> SHMPIQVLPPQLANQIAAGEVVERPASVVKELVENSLDAGATRIDIDIERGGAKLIRIRDNGCGIKKDELALALARHATSKIASLDDLEAIISLGFRGEALASI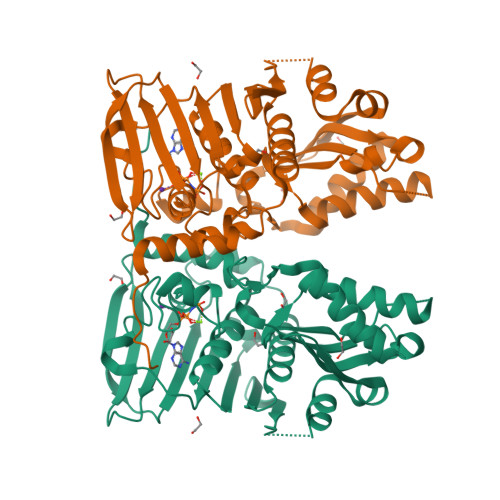SSVSRLTLTSRTAEQQEAWQAYAEGRDMNVTVKPAAHPVGTTLEVLDLFYNTPARRKFLRTEKTEFNHIDEIIRRIALARFDVTINLSHNGKIVRQYRAVPEGGQKERRLGAICGTAFLEQALAIEWQHGDLTLRGWVADPNHTTPALAEIQYCYVNGRMMRDRLINHAIRQACEDKLGADQQPAFVLYLEIDPHQVDVNVHPAKHEVRFHQSRLVHDFIYQGVLSVLQ> GSMASAAVANYEEEIVRPVADFSPSLWGDQFLSFSIKNQVAEKYAKEIEALKEQTRNMLLATGMKLADTLNLIDTIERLGISYHFEKEIDDILDQIYNQNSNCNDLCTSALQFRLLRQHGFNISPEIFSKFQDENGKFKESLASDVLGLLNLYEASHVRTHADDILEDALAFSTIHLESAA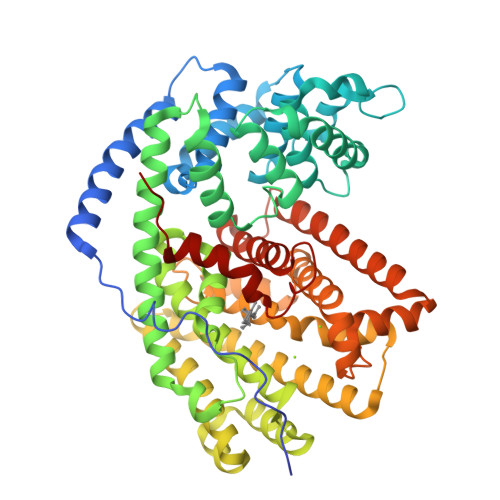PHLKSPLREQVTHALEQCLHKGVPRVETRFFISSIYDKEQSKNNVLLRFAKLDFNLLQMLHKQELAQVSRWWKDLDFVTTLPYARDRVVECYFWTLGVYFEPQYSQARVMLVKTISMISIVDDTFDAYGTVKELEAYTDAIQRWDINEIDRLPDYMKISYKAILDLYKDYEKELSSAGRSHIVCHAIERMKEIVRNYNVESTWFIEGYTPPVSEYLSNALATTTYYLLATTSYLGMKSATEQDFEWLSKNPKILEASVIICRVIDDTATYEVEKSRGQIATGIECCMRDYGISTKEAMAKFQNMAETAWKDINEGLLRPTPVSTEFLTPILNLARIIEVTYIHNLDGYTHPEKVLKPHIINLLVDSIKI> AGALGDAAAAKGRYFGAAVAANHLGEAAYASTLDAQFGSVTPENEMKWDAVESSRNSFSFSAADRIVSHAQSKGMKVRGHTLVWHSQLPGWVSPLAATDLRSAMNNHITQVMTHYKGKIHSWDVVNEAFQDGGSGARRSSPFQDKLGNGFIEEAFRTARTVDADAKLCYNDYNTDGQNAKSNAVYEMVKDFKQRGVPIDCVGFQSHFNSNSPVPSDFQANLQRFADLGVDVQITELDIEGSGSA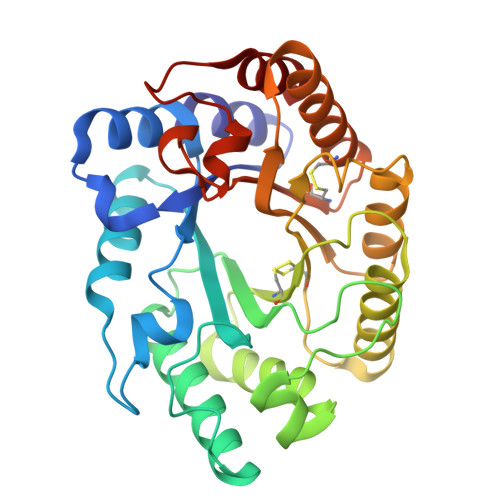QAANYTKVVNACLAVTRCTGITVWGVTDKYSWRSGGTPLLFDGDYNKKPAYDAVLAAL>[2x]DCPSGWSSYEGHCYKPFKLYKTWDDAERFCTEQAKGGHLVSIESAGEADFVAQLVTENIQNTKSYVWIGLRVQGKEKQCSSEWSDG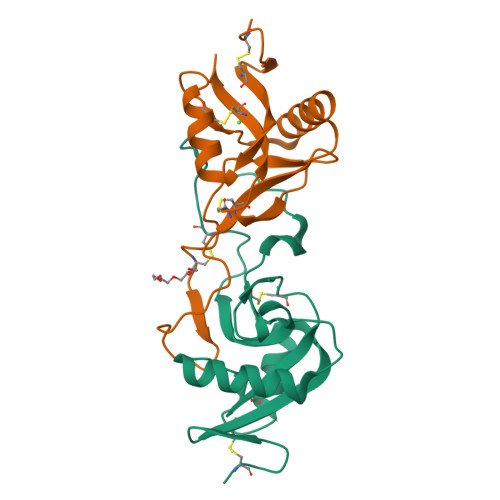SSVSYENWIEAESKTCLGLEKETGFRKWVNIYCGQQNPFVCEA;>[2x]DCPSDWSSYEGHCYKPFSEPKNWADAENFCTQQHAGGHLVSFQSSEEADFVVKLAFQTFGHSIFWMGLSNVWNQCNWQWSNAAMLRYKAWAEESYCVYFKSTNNKWRSRACRMMAQFVCEFQA> KQGPTSVAYVEVNNNSMLNVGKYTLADGGGNAFDVAVIFAANINYDTGTKTAYLHFNENVQRVLDNAVTQIRPLQQQGIKVLLSVLGNHQGAGFANFPSQQAASAFAKQLSDAVAKYGLDGVDFEDEYAEYGNNGTAQPNDSSFVHLVTALRANMPDKIISLYNIGPAASRLSYGGVDVSDKFDYAWNPYYGTWQVPGIALPKAQLSPAAVEIGRTSRST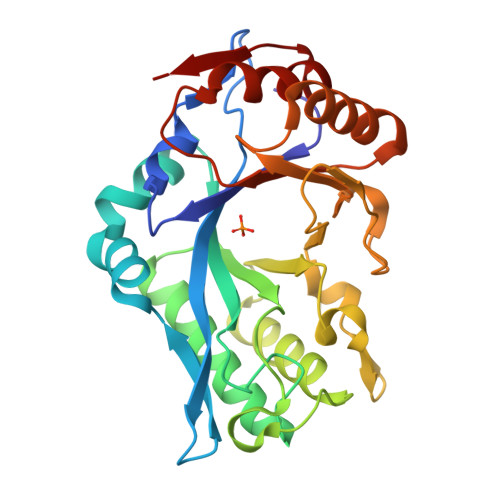VADLARRTVDEGYGVYLTYNLDGGDRTADVSAFTRELYGSEAVRT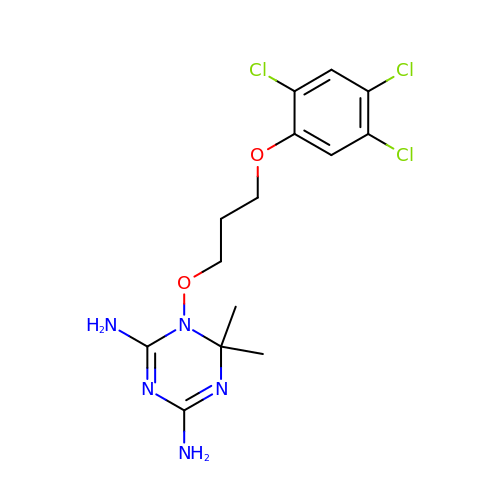6,6-DIMETHYL-1-[3-(2,4,5-TRICHLOROPHENOXY)PROPOXY]-1,6-DIHYDRO-1,3,5-TRIAZINE-2,4-DIAMINE | C14 H18 Cl3 N5 O2 | MJZJYWCQPMNPRM-UHFFFAOYSA-N>[2x]AQLTIEAVPSNAAEGKEVLLLVHNLPQDPRGYNWYKGETVDANRRIIGYVISNQQITPGPAYSNRETIYPNASLLMRNVTRNDTGSYTLQVIK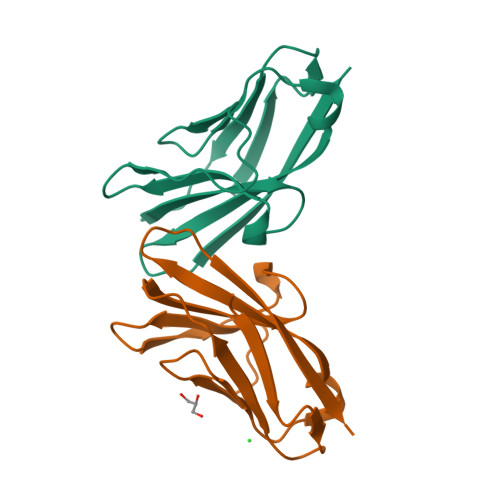LNLMSEEVTGQFSVH;>[2x]AKLTIESTPFNVAEGKEVLLLAHNLPQNRIGYSWYKGERVDGNSLIVGYVIGTQQATPGPAYSGRETIYPNASLLIQNVTQNDTGFYTLQVIKSDLVNEEATGQFHVY> PMHPFVKALQEHFTAHQNPEKAEPMARYMKNHFLFLGIQTPERRQLLKDIIQIHTLPDQKDFQIIIRELWDLPEREFQAAALDIMQKYKKHINETHIPFLEELIVTKSWWDSVDSIVPTFLGDIFLKHP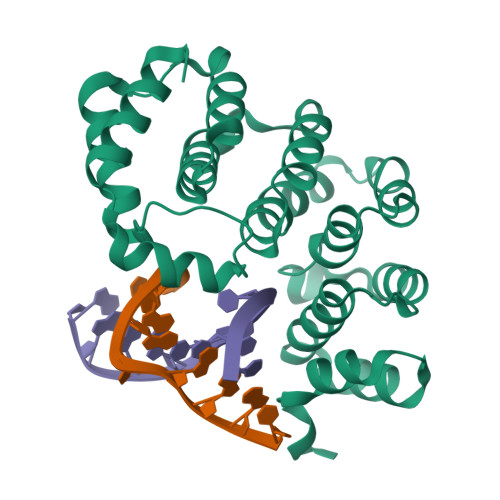ELISAYIPKWIASDNIWLQRAAILFQLKYKQKMDEELLFWIIGQLHSSKEFFIQKAIGWVLREYAKTNPDVVWEYVQNNELAPLSKREAIKHIKQNY>MDGIAELTGARVEDLAG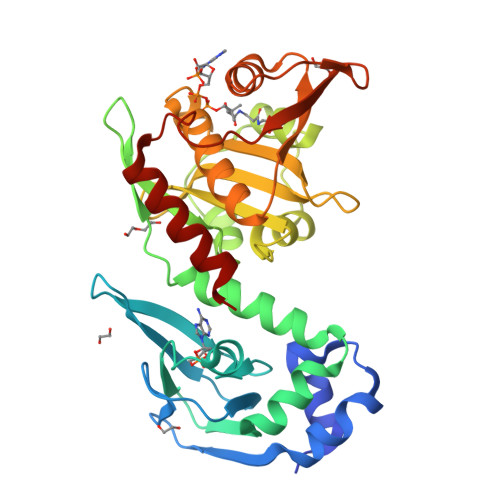MDVFQGCPAEGLVSLAASVQPLRAAAGQVLLRQGEPAVSFLLISSGSAEVSHVGDDGVAIIARALPGMIVGEIALLRDSPRSATVTTIEPLTGWTGGRGAFATMVHIPGVGERLLRTARQRLAAFVSPIPVRLADGTQLMLRPVLPGDRERTVHGHIQFSGETLYRRFMSARVPSPALMHYLSEVDYVDHFVWVVTDGSDPVADARFVRDETDPTVAEIAFTVADAYQGRGIGSFLIGALSVAARVDGVERFAARMLSDNVPMRTIMDRYGAVWQREDVGVITTMIDVPGPGELSLGREMVDQINRVARQVIEAVG[2x]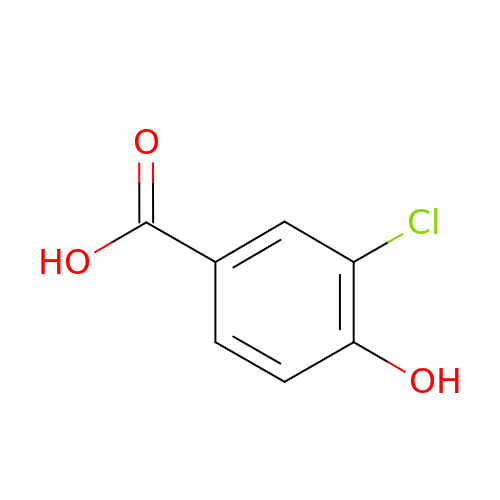3-CHLORO-4-HYDROXYBENZOIC ACID | C7 H5 Cl O3 | QGNLHMKIGMZKJX-UHFFFAOYSA-N>MSFFDLLNERAKRSLLCVGLDPRAKTAAAAVEECKRLIEQTHEYAAAYKPNAAFFEFFGAEGWAALSEVIRAVPAGIPVVLDAKRGDIADTADAYATSAFKHLNAHAITASPYMGSDSLQPFMRYPDKAVFVLCKTSNKGSNDLQCLRVGDRYLYEAVAERAEGPWNVNGNVGLVVGATDPVALARVRARAP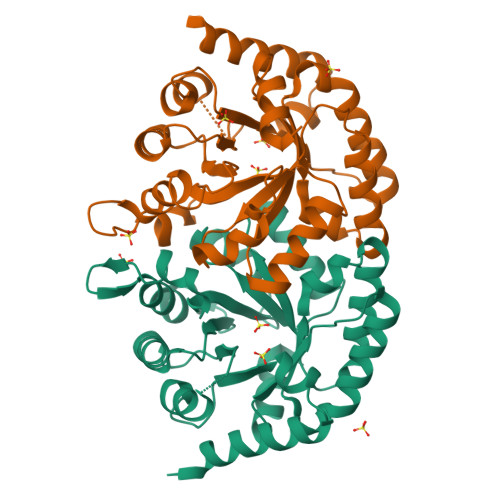TLWFLVPGIGAQGGSLKASLDAGLRADGSGMLINVSRGLARAADPRAAAKELCEEINAIRFAA[2x]> KNRSLSVRVSTFDSELEFKLEPRASGQDLFDLVCRTIGLRESWYFGLQYVDTRSNVSWLKMEKRVRDQRVELHASNNVYVFSFYAKFFPENVSEELIQEITQHLFFLQVKQSILSMDIYCRPEASVLLASYAVHVQYGPYDYETYKDGMLAGGELLPKGVTDQYQMTPEMWEERIKTWYMDHEPMTRDEVEMEYLKIAQDLDMYGVNYFP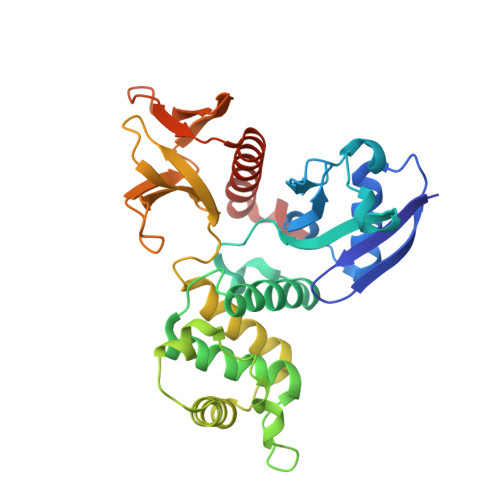ITNKNKTKLWLGVTSVGLNIYDERDKLTPKTTFQWNEIRHVSFDDKKFTIRLVDAKVSNFIFYSQDLHINKMILDLCKGNHDLYMRRRKPDTMEIQQ> MSGFSLSEYLTKFQTTDRESYPRLQDPSRELNVIIDQLAVSPEQIDASPDSLEALIDLCHDFPHLTPKLQTQLSYLISSSLSNLSKDIKANLSSNVNFTEIGGLIPQWKRHLEEYGYLIQVLLTFLQDELHKVSSQSTNLNRSAKNSKNDSANVELFKRDCNQMENLLESITKLLEINLSKIFQTTPEKDLFIGLFTRPLFVLLEIEPVTKVSSLKMFIQRILAMCVKNHGQSSSIQSSLMTNLTYFLHLSVFNAELLKLLNDEYNYPQLTEDILKEISTRVFNAKDTTGPKAISNFLIKLSELSPGIMLRQMNLVITLLNNSSITLRCSVVEACGNIVAELAQDPQTMEHYKQQIAVLIELLEERFQDSNPYVRTKAIQGCSKICDLSSKFNKSKAKFTSLAVRSLQDRSSLVRRNSVKLLSKLLLKHPFKAIHGSQLRLSEWEEYLKGSESQLNSTLKKVESQETLNDTIERSLIEEEVEQDEGQCRTELEGSFNKSAELSRIENEVENINATNTSVLMKLKLMIVYYKDAISFIKEIHKSIELISNLLFSKNRNEVLESMDFLVLADAFDIELSEFGIKKMLHLVWMKGTNDEGTSISVHLIECYKQLFLTAPDSCNMQEKAAHIAKNLINLSIGASIADLASLEQLLGMMYEQKLIDQHVINILWAIYNSASKASMQKEQNVNNRDSEKGFSKEQIHGSIIILGMLSLADNEIALKGLESLLNIGLGAVGLKDLTLCRYSCLALERMVPKRSTIITKAINQELEDVAVKKLYAIIINYTKDNEYYPMCEQALSALFTISSKPDILATDLIREKTMMTFGKPEEEDSILSLEQSSRVVSLSQLLFIVGQVAIKTLVYLEKCEAEFKKRKIEAETRNGKVKNQGADVTNTTQDNGGDKELEMIGGTNEDDFTDAIQFVKENELLFGEKSILGKFCPIVEEIVSNSSRFSDPMLQRTATLCLEKLMCLSSKYCEKSLPLLITVMEKSPDPTIRSNAVLGLGDMAVCFNNLVDENTDYLYRRLHDENLMVQRTCLMTVTFLIL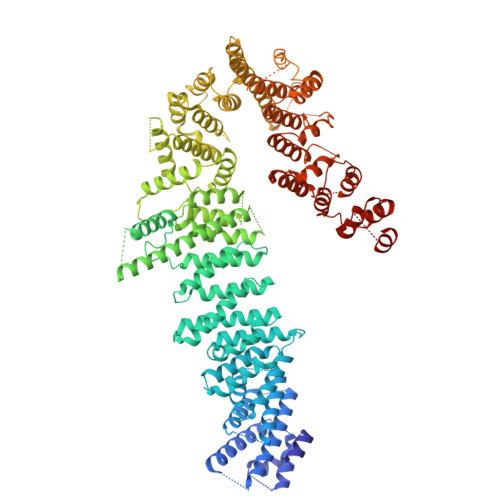AGQVKVKGQLGEMAKCLDNPDQGISDMCRLFFTELASKDNAIYNGFIDIFSNLSSDDLLGKESFKKIIKFLLTFIDKERHQKQLNEKLVGRLRKCETQKQWDDIAFVLNNLPYKNEDVTALLEQGFKVVSAKEXXXXXXXXX>[2x]MVSGFAMPKIWRKLAMDIPVNAAKPGRRRYLTLVMIFITVVICYVDRANLAVASAHIQEEFGITKAEMGYVFSAFAWLYTLCQIPGGWFLDRVGSRVTYFIAIFGWSVATLFQGFATGLMSLIGLRAITGIFEAPAFPTNNRMVTSWFPEHERASAVGFYTSGQFVGLAFLTPLLIWIQEMLSWHWVFIVTGGIGIIWSLIWFKVYQPPRLTKGISKAELDYIRDGGGLVDGDAPVKKEARQPLTAKDWKLVFHRKLIGVYLGQFAVASTLWFFLTWFPNYLTQEKGITALKAGFMTTVPFLAAFVGVLLSGWVADLLVRKGFSLGFARKTPIICGLLISTCIMGANYTNDPMMIMCLMALAFFGNGFASITWSLVSSLAPMRLIGLTGGVFNFAGGLGGITVPLVVGYLAQGYGFAPALVYISAVALIGALSYILLVGDVKRVGSLVPRGSGSHHHHHH

Members of the solute carrier 17 (SLC17) family catalyze the coupled transport of anions driven by a proton electrochemical gradient ΔμH+ (= Δψ − 2.3× (RT/F) × ΔpH, where R is the gas constant, T is temperature, and F is Faraday’s constant), with contributions from both electrical potential Δψ and proton gradient ΔpH (pHo/pHi). The D-galactonate transporter (DgoT) gene lies within an operon devoted to the metabolism of D-galactonate, suggesting a role in transport of this acidic sugar. DgoT is composed of 12 TM helices and belongs to the MFS fold. Two 6-helix bundles (N- and C-terminal domains) are related by a pseudo 2-fold symmetry axis perpendicular to the membrane plane.

To determine the structure of DgoT, the wild type (WT) protein was crystallized at pH 5.35, in an inward-open conformation and crystal space group P21. Nonsubstrate gluconate improved the diffraction, and it as well as β-nonylglucoside (β-NG) were identified nonspecifically within the aqueous cavity of the structure. The structure was determined to a resolution of 2.9 × 3.8 × 3.8 Å by molecular replacement (MR) trials based on all available major facilitator superfamily (MFS) transporters in turn because the MFS typically each crystallize in different parts of the transport cycle. The asymmetric unit contains 2 almost identical, antiparallel monomers of DgoT, with 4 molecules of β-nonylglucoside (β-NG) between the 2 molecules of DgoT and a root-mean-square deviation (rmsd) of 0.57 Å between their congruent 392 Cα atoms. The structure contains residues 27 through 443, lacking a 6–amino acid unstructured cytoplasmic loop (residues 235–242) between transmembrane (TM) domains 6 and 7. Although the main cavity of the inwardly oriented structure is sealed to the outside, the N-terminal lobe of DgoT contains a tunnel that extends from the periplasmic surface near glutamate-180 (Glu180; TM5) to a membrane-embedded site at aspartate-46 (Asp46; TM1). Polar residues lining the entrance (Glu59, glutamine-179 [Gln179], Glu180), interior (threonine-172 [Thr172], Thr297), and exit (Asp46) have the potential to interact with H3O+ and could therefore facilitate H+ transport. On the other hand, residues phenylalanine-278 (Phe278), proline-279 (Pro279), and Thr297 reduce the tunnel diameter to 2.4 Å, about the diameter of a water molecule (2.75 Å), suggesting a dynamic mechanism to control access of H3O+ from the periplasm. Thus, Asp46 is most probably protonated (uncharged) in this structure. In the inward-facing conformation, TM4 is continuous, whereas TM10 has a kink.>[2x]MSQLDLLNIVHRPRRLRRTAALRNLVQENTLTVNDLVFPLFVMPGTNAVEEVSSMPGSFRFTIDRAVEECKELYDLGIQGIDLFGIPEQKTEDGSEAYNDNGILQQAIRAIKKAVPELCIMTDVALDPFTPFGHDGLVKDGIILNDETVEVLQKMAVSHAEAGADFVSPSDMMDGRIGAIREALDETDHSDVGILSYAAKYASSF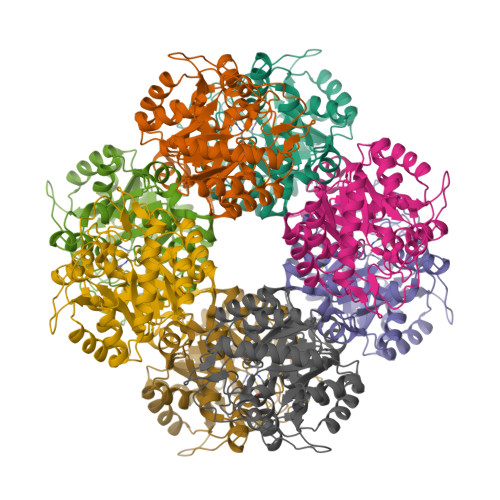YGPFRDALHSAPQFGDKSTYQMNPANTEEAMKEVELDIVEGADIVMVKPGLAYLDIVWRTKERFDVPVAIYHVSGEYAMVKAAAAKGWIDEDRVMMESLLCMKRAGADIIFTYYAKEAAKKLR> SMQAEVLLQPDFNAEKFSGLWYVVSMASDCRVFLGKKDHLSMSTRAIRPTEEGGLHVHMEFPGADGCNQVDAEYLKVGSEGHFRVPALGYLDVRIVDTDYSSFAVLYIYKELEGALSTMVQLYSR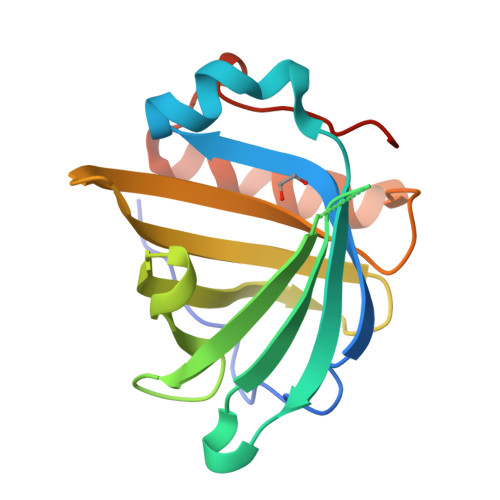TQDVSPQALKSFQDFYPTLGLPKDMMVMLPQSDACN>MNVKETKLEDVLKSRGIDMKDAYNISEADIPEAKESTQKLMDIYYTLKVTADMEAAYWYNRTWWENDGEVIEVRRAKAVAASLSHMTPTILPYEKLVMNKTKNVRGAFPFPWVCASFFNAQAEALMNEVDAPAENEADSVSVVGAGGGNVTESYGNVISIAKKFGMRKEEIPVLVKTSKPWEGISVEELSNKYSKMTPGYDQFKNIMESVICMFDSFAIPQGREVINYYMPLQYGFDGIIKLCDEKIAEVMGEAGDDGDFGMSRGYYYAAMKEITKGLSAWCENYSKRAKYLASIETDSEIKANYEKIEEVMGNIAHKKPANFWEAIQMTLCCHFGVVNEDPQSGLSIGRLGQVLQPFYEKDVEDGIMTDEEVIELLELYRIKITCIECFASAGVSGGVLSGNTFNNLSLGGQNYDGLSAVTPLEYLIVEAGMRNQTPQPTLSVLYDEKTPEDFLMKAASCTKLGLGYPAWMNNQTGMNFMMRNYGPEGMDLHDARAWCLGGCLESAPGCFLPLEYNGKVTMIPGGASPTCGTGVHFIGMPKVLELVLTNGLDKRTGKQVYPPHNKKLDSYETMVNQWKEYMELTTDVVNRCNNIQMDIWRKYNMPAVNSLLKPDCFKKGKHIGTMGARYNSCINFESCGTITFVNSLSSIKKNVFDDSKFTIEEMT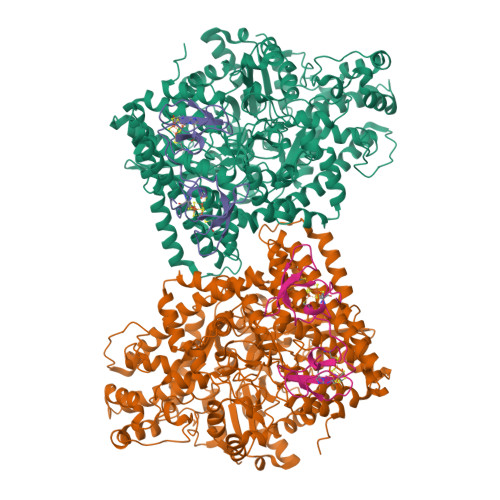DAMLNNFGFKTAYETEVFSPDFRESTDKSTKYEKIFAACVNAPKYGNADKYADEIFKAYHYYIYDMTHKFRSYYGKPLYLCQISVSTHGPQGFVTLATADGRLAGTTYSDGSVSAAAGTDKNGIYAIFESATVYDHSMHQNAQMNLKLHPTAVKGINGTRKLLDLVRAYMRKGGFHVQFNVVDSKTLRDAQLTPEKYRELMVRVAGFTQYWCEIGKPIQDEVIYRTEYDK[2x];>MRHYDCKNYINLDCEKGLCALTKGMVPIDGEGSEACPNFKPAEKCGNCKNFCNPDKYGLGTCTGLEKENWAYATCGASACPSYKAE[2x]> MAHAGRTGYDNREIVMKYIHYKLSQRGYEWDAGDDVEENRTEAPEGTESEVVHLTLRQAGDDFERRYRR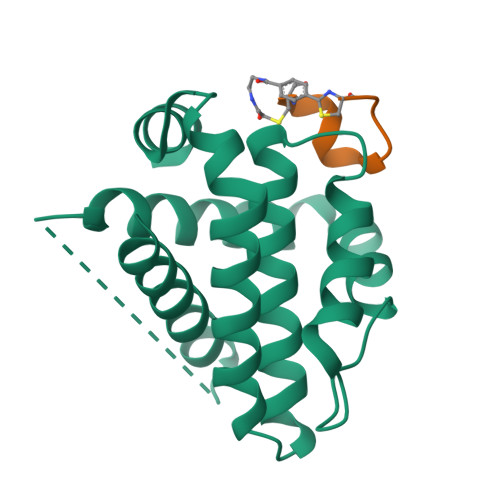DFAEMSSQLHLTPFTARGRFATVVEELFRDGVNWGRIVAFFEFGGVMCVESVNREMSPLVDNIALWMTEYLNRHLHTWIQDNGGWDVFVELYGPSMR;> CPARYGWDYECX> GPSQDASDGLQRLHMLQISYFRDPYHVWYQGNASLGGHLTHVLEGPDTNTTIIQLQPLQEPESWARTQSGLQSYLLQFHGLVRLVHQERTLAFPLTIRCFLGCELPPEGSRAHVFFEVAVNGSSFVSFRPERALWQADTQVTSGVVTFTLQQLNAYNRTRYELREFLEDTCVQYVQKHISAENTKGSQTSRSYTS

EPCR is a transmembrane MHC class I-like glycoprotein primarily abundant in the vasculature of large vessels, but present in numerous cell types. Since its identification, EPCR has been mainly known for its role in accelerating the generation of the anticoagulant activated protein C (APC) and favoring its cytoprotective properties. Structurally, EPCR shares a notable degree of homology with the CD1 family of receptors, including the presence of a central and extended hydrophobic cavity suitable for lipid antigens, flanked by two alpha helices lying on top of a beta sheet. The presence of a lipid bound to EPCR is key for its biological functions.

In the delipidated EPCR structure, the electron density for the Arg156 side chain is absent, which suggests high flexibility (elevated B-factors) and conformational disorder. Moreover, and in line with the lipid dependency of EPCR, surface plasmon resonance studies showed that loading of delipidated EPCR, whose interaction with protein C/APC is compromised, with PC restored its binding ability.>[2x]MAHHHHHHSSGLEVLFQGPMNRTCMAMPYFEIPERHLEAFKAYCAVFIEKTSKEPGCLYYGFSFNGTQGHCREVYSDAQGLLNHLVNIAELNSEAFHLASIVRYEVHGPREELDK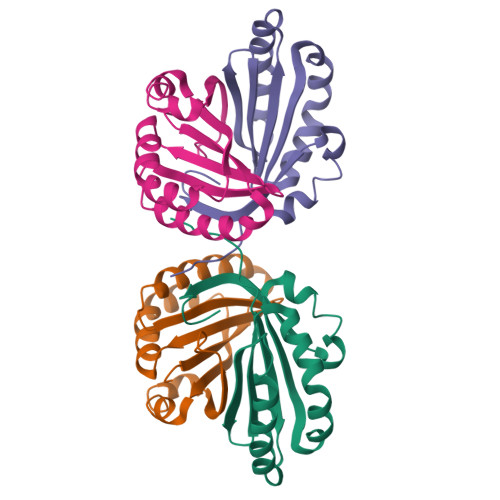LRGPLAFMKPQFFELEQCFSRPSVVA> MAGWQSYVDNLMCDGCCQEAAIVGYCDAK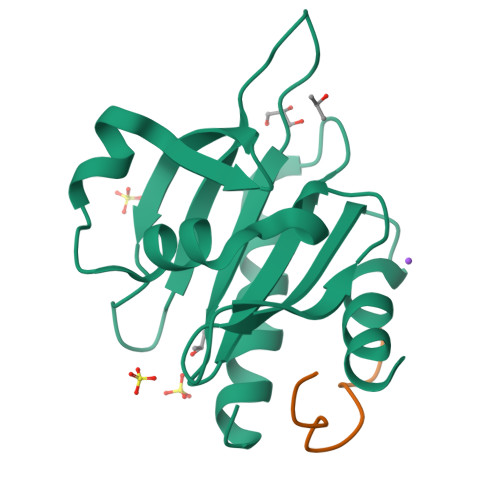YVWAATAGGVFQSITPVEIDMIVGKDREGFFTNGLTLGAKKCSVIRDSLYVDGDCTMDIRTKSQGGEPTYNVAVGRAGRVLVFVMGKEGVHGGGLNKKAYSMAKYLRDSGF;> GPPPPPGPPPPPGPPPPPGL> GDVVEAIEGAVARVADTISSGPTNSQAVPALTAVETGHTSQVVPGDTMQTRHVKNYHSRSESTIENFLSRSACVYMGEYYTTNTDETKRFASWTINARRMVQMRRKLEMFTYVRFDVEVTFVITSKQDQGTQLGQDMPPLTHQIMYIPPGGPIPKSTTDYAWQTSTNPSIFWTEGNAPPRMSIPFVSIGNAYSNFYDGWSHFSQNGVYGYNTLNNMGQLYMRHVNGPSPLPMTSIVRVYFKPKHVKAWVPRPPRLCQYKNASTVNFSSTNITDKRDSITHVPDTVKPDVTTH;> SPSAEECGYSDRVRSITLGNSTITTQECANVVVAYGRWPEYLSDKEATAEDQPTQPDVATCRFYTLESVTWEKDSPGWWWKFPDALKDMGLFGQNMYYHYLGRAGYTIHVQCNASKFHQGCLLVVCVPEAEMGCSDVGGTVNEHAISEGEIAKKFSATATNGAHTVQSIVTNAGMGVGVGNLTIYPHQWVNLRTNNSATIVMPYINSVPMDNMFRHHNFTLMIIPFVSLDYSSDASTYVPITVTVAPMCAEYNGLRLATSLQ;> GLPVMNTPGSNQFLTSDDFQSPSAMPQFDVTPELDIPGEVKNLMEIAEVDSVVPVNNVVGKLDTMDIFRIPVQSGNHQSTQVFGFQVQPGLDSVFKHTLLGEILNYYAHWSGSVKLTFVFCGSAMATGKFLLAYSPPGANAPKTRKDAMLGTHVIWDVGLQSSCVLCIPWISQTHYRLVHQDEYTSAGNVTCWYQTGIVVPAGTPTLCSIMCFVSACNDFSVRLLKDTPFIEQSALLQ;> MGAQVSTQKTGAHETGLNASGNSIIHYTNINYYKDAASNSANRQDFTQDPGKFTEPVKDIMIKSMPALN;> MGCVAETGDCGLPPDVPNAQPALEGRTSFPEDTVITYKCEESFVKIPGEKDSVICLK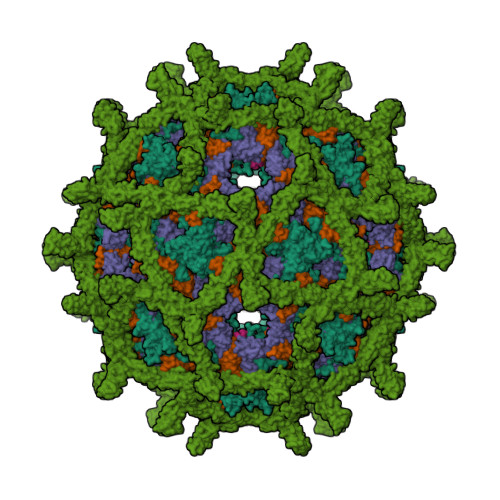GSQWSDIEEFCNRSCEVPTRLNSASLKQPYITQNYFPVGTVVEYECRPGYRREPSLSPKLTCLQNLKWSTAVEFCKKKSCPNPGEIRNGQIDVPGGILFGATISFSCNTGYKLFGSTSSFCLISGSSVQWSDPLPECREIYCPAPPQIDNGIIQGERDHYGYRQSVTYACNKGFTMIGEHSIYCTVNNDEGEWSGPPPECRGGTKHHHHHH> GPLGSWSWESYLEEQKAITAPVSLFQDSQAVTHNKNGFKLGMKLEGIDPQHPSMYFIL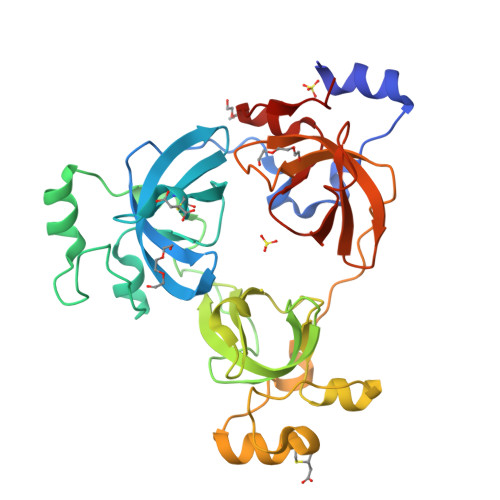TVAEVCGYRLRLHFDGYSECHDFWVNANSPDIHPAGWFEKTGHKLQPPKGYKEEEFSWSQYLRSTRAQAAPKHLFVSQSHSPPPLGFQVGMKLEAVARMNPSLVCVASVTDVVDSRFLVHFDNWDDTYDYWCDPSSPYIHPVGWCQKQGKPLTPPQDYPDPDNFCWEKYLEETGASAVPTWAFKVRPPHSFLVNMKLEAVDRRNPALIRVASVEDVEDHRIKIHFDGWSHGYDFWIDADHPDIHPAGWCSKTGHPLQPPLG We present a study of the amino-terminal segment of MUC5AC, one of the two main respiratory mucins. Though normally produced at lower levels than MUC5B, which is the dominant mucin in healthy lungs, MUC5AC is induced upon infection, and high MUC5AC levels are protective against respiratory viruses. In this work, the high-resolution structures obtained for two helical filamentous forms of MUC5AC, determined by cryoelectron microscopy (cryo-EM), are described. The structures of MUC5AC helical filaments also strengthen the generality of the bead-based mechanism for bringing D3 assemblies together for disulfide bonding and polymer formation.

In addition to the filament maps, a single-bead map was obtained at 2.9 Å resolution. An atomic coordinate model for a single bead was refined, and the resulting structure was docked into the two-start helix map and replicated using the helical parameters to provide a helix model. Within each MUC5AC bead, two copies of the D1 and D2 segment, arranged antiparallel to one another, cradle the central pair of disulfide-bonded D3 assemblies, as in MUC2 and VWF. The two interacting D3 assemblies in MUC5AC are connected to the D1 and D2 segments from the two neighboring beads through interbead bridges composed of the TIL2/E2/TIL2′/E′ domains, as also seen for the related proteins. MUC5AC is more compact than MUC2, smaller by about 8 Å in both the long and the short axes of the oblong bead. The MUC5AC VWD1 domain contacts both the VWD3 domain, located near the edge of the bead, and the C8-3 domain, located near the center of the bead. A further interaction observed in MUC5AC was a segment of polypeptide upstream of the VWD1 domain participating in an intermolecular β-sheet by hydrogen bonding to an exposed β-strand in VWD3. TIL3 was the last domain that could be modeled from the MUC5AC cryo-EM density. In the MUC5AC cryo-EM structures, side chain nitrogens of the three histidines in the putative Cu2+ binding site were seen at distances of about 2.1 Å from a central density, which appeared at 14σ in the bead map. Density for the glutamate carboxylate was ambiguous, but 6σ map density clearly showed the side chain oriented toward the histidines and their metal ligand.

>[4x]QDGSSESSYKHHPALSPIARGPSGVPLRGATVFPSLRTIPVVRASNPAHNGRVCSTWGSFHYKTFDGDVFRFPGLCNYVFSEHCGAAYEDFNIQLRRSQESAAPTLSRVLMKVDGVVIQLTKGSVLVNGHPVLLPFSQSGVLIQQSSSYTKVEARLGLVLMWNHDDSLLLELDTKYANKTCGLCGDFNGMPVVSELLSHNTKLTPMEFGNLQKMDDPTDQCQDPVPEPPRNCSTGFGICEELLHGQLFSGCVALVDVGSYLEACRQDLCFCEDTDLLSCVCHTLAEYSRQCTHAGGLPQDWRGPDFCPQKCPNNMQYHECRSPCADTCSNQEHSRACEDHCVAGCFCPEGTVLDDIGQTGCVPVSKCACVYNGAAYAPGATYSTDCTNCTCSGGRWSCQEVPCPGTCSVLGGAHFSTFDGKQYTVHGDCSYVLTKPCDSSAFTVLAELRRCGLTDSETCLKSVTLSLDGAQTVVVIKASGEVFLNQIYTQLPISAANVTIFRPSTFFIIAQTSLGLQLNLQLVPTMQLFMQLAPKLRGQTCGLCGNFNSIQADDFRTLSGVVEATAAAFFNTFKTQAACPNIRNSFEDPCSLSVENEKYAQHWCSQLTDADGPFGRCHAAVKPGTYYSNCMFDTCNCERSEDCLCAALSSYVHACAAKGVQLGGWRDGVCTKPMTTCPKSMTYHYHVSTCQPTCRSLSEGDITCSVGFIPVDGCICPKGTFLDDTGKCVQASNCPCYHRGSMIPNGESVHDSGAICTCTHGKLSCIGGQAPAPVCAAPMVFFDCRNATPGDTGAGCQKSCHTLDMTCYSPQCVPGCVCPDGLVADGEGGCITAEDCPCVHNEASYRAGQTIRVGCNTCTCDSRMWRCTDDPCLATCAVYGDGHYLTFDGQSYSFNGDCEYTLVQNHCGGKDSTQDSFRVVTENVPCGTTGTTCSKAIKIFLGGFELKLSHGKVEVIGTDESQEVPYTIRQMGIYLVVDTDIGLVLLWDKKTSIFINLSPEFKGRVCGLCGNFDDIAVNDFATRSRSVVGDVLEFGNSWKLSPSCPDALAPKDPCTANPFRKSWAQKQCSILHGPTFAACHAHVEPARYYEACVNDACACDSGGDCECFCTAVAAYAQACHEVGLCVSWRTPSICPLFCDYYNPEGQCEWHYQPCGVPCLRTCRNPRGDCLRDVRGLEGCYPKCPPEAPIFDEDKMQCVATCPTPPLPPRCHVHGKSYRPGAVVPSDKNCQSCLCTERGVECTYKAEACVCTYNGQRFHPGDVIYHTTDGTGGCISARCGANGTIERRVYPCSPTTPVPPTTFSFSTPPLVVSSTHTPSNGPSSAHTGPPSSAWPTTAGTSPRTRLPTASASLPPVCGEKCLWSPWMDVSRPGRGTDSGDFDTLENLRAHGYRVCESPRSVECRAEDAPGVPLRALGQRVQCSPDVGLTCRNREQASGLCYNYQIRVQCCTPLPCST The generic transketolase (EC 2.2.1.1; Tkt) is a ubiquitous enzyme that catalyses the cleavage of a carbon–carbon bond adjacent to a carbonyl group of a ketose sugar and transfers a two-carbon moiety to an aldose sugar. A cofactor, thiamine pyrophosphate (TPP), and a divalent metal ion, Mg2+ by preference, are required for catalysis. More specifically, megaplasmid-encoded transaldolase (LSL_1888, mipB) and transketolase (LSL_1946, tktA) complete the pentose phosphate pathway of L. salivarius UCC118. In this work, we present high-resolution crystal structures of the L. salivarius UCC118 Tkt protein (LsTktA) in the presence and absence of the cofactor TPP and Mg2+ ions, which have been determined as part of a directed structural genomics approach to furthering our understanding of how these bacterial strains colonize and persist in the human gut and enhance the wellbeing of the host.

LsTktA crystallizes in the trigonal space group P3221 with a protomer in the asymmetric unit. Overall, apo-monomer dimerization buries an interface area of 3998 Å2 of each subunit with the formation of 16 salt bridges, 60 hydrogen bonds and numerous hydrophobic interactions predominantly involving residues from the first two domains of each monomer (residues 1–528). Two peaks corresponding to molar masses (MWs) of 138.8 (±0.8) and 70.4 (±2.4) kDa were observed for the apo protein, corresponding closely to the theoretical dimeric and monomeric MWs calculated from the amino-acid sequence of the histidine-tagged Tkt, which consists of 680 amino acids. The peak distribution indicated approximately 75% dimeric and 25% monomeric species in solution. Other changes involve small shifts in the loop 190–198, which is clearly resolved in both structures. This differs from the structure of S. cerevisiae Tkt, where two flexible loops (region 185–198 and 383–393) could not be modelled owing to an absence of electron density in the apo structure. In comparison to the apo structure, 48 of the 54 superpositions had a global r.m.s.d. of less than 2 Å, with the largest r.m.s.d.s (∼7 Å) observed for the human Tkt structures. The two structures are globally very similar, with some slight side-chain rearrangements triggered by cofactor binding.

> MAHHHHHHSSGLEVLFQGPYDQVDQLGVNTLRTLSIDAIQRANSGHPGLPMGAAPMAYVLWTRHLKINPKTHMNWVNRDRFVLSAGHGSALLYSLAHLAGYDVSMDDLKNFREWKSNTPGHPEYGCTDGVEATTGPLGQGISMAVGMAMAEAHLGKKFNREGYPVMDHYTYALIGDGDLMEGVASEAASLAGHLKLGKLIALYDSNGISLDGKTSASFTENVGARFEAYGWQYILVEDGFNLEEIDKAIVQAKAESDKPTIIEIKTTIGYGSENQGTHKVHGSPLGEEGVAHAKEVYNWNYPPFTVPEEVSQRFKECLQDKGVKAENKWNEMFEAYKKEYSDLAQKFSDGFSNKVPNTLGDILPQYGEDDSIATRAASQKAINALAKEVSSLWGGAADLASSNKTVIAGEGDFQPESYEGRNIWFGVREFGMACAMNGIMLHGGTRIFGSTFFVFSDYLKAAIRLSAIQKLPVIYVLTHDSVAVGKDGPTHEPIEQLASLRTIPNVQVFRPADGNETSAAWKVALETLDKPTILVLSRQNLDTLPISKEKVFDGVEKGGYVVQGAENEADGILIATGSEVGLALKAKEELQKKGKDVIVVSLPSWERFEAQSEEYKNTVIPPELKKRMTIEAGTTYGWAKYAGDHGVMIGIDEFGMSAPSDIVLRELGMSVENIVDKYLEK iodobenzene 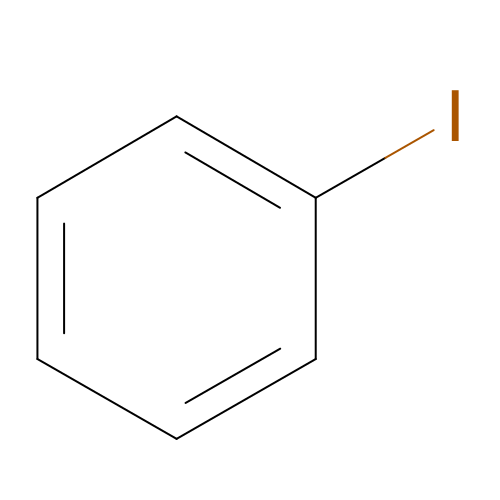| C6 H5 I | SNHMUERNLJLMHN-UHFFFAOYSA-N>[3x]MRKVLGVLAGLVLGIPGVAAERHFTLEARSSIFEVDQGVYLRGFSFNDMSPGPMLVVEEGDTVHITLRNLDNVTHGLSIHAANTQTSRFLGNVQPGETREFSFTADFPGVFMYHCAPGGHGIMAHTMGGQFGMIVVEPKEKYRMERELGRGPDLKLYIIQSEAYASGRDFYDGKALYVMFNGRNFRYVDEPIPVRPGDYLRIYFLNVGPNLTSTLHVVGGIFEYMYYQGNPKNLVVGAQTALAGPSDSWVIEWRVPPVEGDYTLVTHVFGTAIKGALGILRAKKDAPRIPEVRAEGVPGVKEIPASAKRVVDPYGLASPGHEHTVRVPLDPALAQPVAVGAKALEPLPVTVQMVGNSFYPKVLEIPVGTTVEFVNEDVFDLLEGERTGRHDAVVIDVQGPEPFVTPKLGHGERYRITFTKPGEYVYICSIHPYMKGIIRVYEPLSQRADSQ

Here we describe the crystal structure of the NirK from T. scotoductus SA-01 (TsNirK) at a resolution of 1.63 Å together with its biochemical and spectroscopic characterization. TsNirK is a homotrimer with subunits of 451 residues that contain three copper atoms each. The N-terminal region possesses a type 2 Cu (T2Cu) and a type 1 Cu (T1CuN) while the C-terminus contains an extra type 1 Cu (T1CuC) bound within a cupredoxin motif.

However, a single crystal was obtained that indexed to C121, containing the entire homotrimer in the ASU. The characteristic extra loop (Asn181–Pro191) and the tower loop (Tyr164–Leu176) of two-domain NirKs were observed within domain II. Domains I and III harbour the copper centres [Fig. 2(b)] and a calcium atom from the crystallization solution, coordinated by residues of domain I, is found between the monomers. T1CuN is located at the top of domain I and is coordinated by two His Nδ1 residues (His75 and His125), Cys115 Sδ, and a Gln130 O∊1 residue in apical position. T1CuC is an amicyanin-like T1Cu centre with the His2 Nδ1–Cys Sδ–Met Sγ ligand set and an additional carbonyl O atom from Arg389 trans to the axial Met ligand. Structural data for TsNirK suggest a potential electron-transfer pathway of T1CuC → T1CuN → T2Cu as there is no exposed hydrophobic patch through which a physiological external electron donor can potentially interact directly with the T1CuN centre. The most likely T1CuC → T1CuN electron-transfer route would involve domains I and III within the same subunit [Figs. 2(d) and S3]; in this pathway T1CuC might deliver electrons via a hydrogen-bonded His431 N∊2–wat–Glu385 O∊1–His125 N∊2 chemical path to the T1CuN centre.> MPYAGSELPRRPLPPAAQERDAEPRPPHGELQYLGQIQHILRCGVRKDDRTGTGTLSVFGMQARYSLRDEFPLLTTKRVFWKGVLEELLWFIKGSTNAKELSSKGVK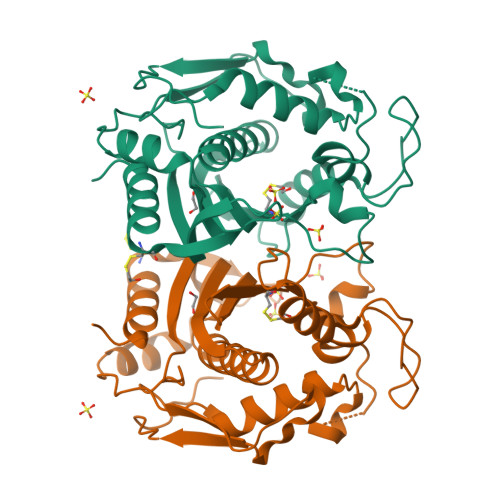IWDANGSRDFLDSLGFSTREEGDLGPVYGFQWRHFGAEYRDMESDYSGQGVDQLQRVIDTIKTNPDDRRIIMCAWNPRDLPLMALPPCHALCQFYVVNSELSCQLYQRSGDMGLGVPFNIASYALLTYMIAHITGLKPGDFIHTLGDAHIYLNHIEPLKIQLQREPRPFPKLRILRKVEKIDDFKAEDFQIEGYNPHPTIKMEMAV>[4x]MAHHHHHHMSRQRPVALVTGGRRGIGLG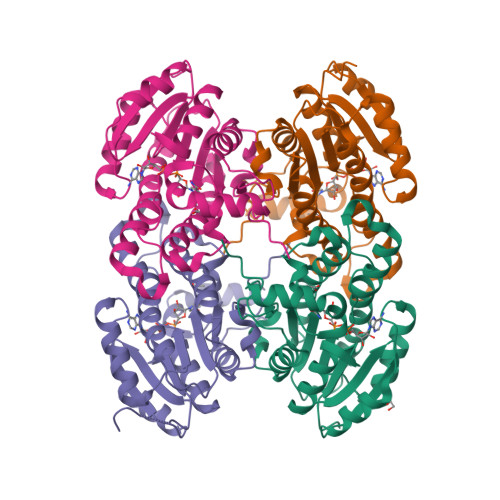IARALAAKGFDLAITDRESDEAVIHELRGLGGKVAFFKSDLAAVKTHEATVFAVLDAFGGIDCLVNNAGMGAVERGDFLALKPENFDTIMDVNLRGTVFFTQAVVKAMLAADEVRFPRSIVTISSVSSVMTSPERLDYCISKAGLTAFVQGLALRLAEARIGVFEVRPGIIRTDMTAKVAARYDALIEGGLVPMKRWGEASDVGAIVAGLAGGDFIFATGSAIHADGGLSIAKL> SRAPDQDEIQRLPGLAKQPSFRQYSGYLKGSGSKHLHYWFVESQKDPENSPVVLWLNGGPGCSSLDGLLTEHGPFLVQPDGVTLEYNPYSWNLIANVLYLESPAGVGFSYSDDKFYATNDTEVAQSNFEALQDFFRLFPEYKNNKLFLTGESYAGIYIPTLAVLVMQDPSMNLQGLAVGNGLSSYEQNDNSLVYFAYYHGLLGNRLWSSLQTHCCSQNKCNFYDNKDLECVTNLQEVARIVGNSGLNIYNLYAPCAGGVPSHFRYEKDTVVVQDLGNIFTRLPLKRMWHQALLRSGD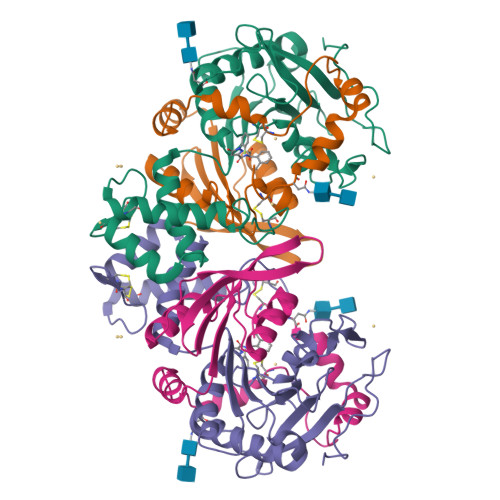KVR;> MDPPCTNTTAASTYLNNPYVRKALNIPEQLPQWDMCNFLVNLQYRRLYRSMNSQYLKLLSSQKYQILLYNGDVDMACNFMGDEWFVDSLNQKMEVQRRPWLVKYGDSGEQIAGFVKEFSHIAFLTIKGAGHMVPTDKPLAAFTMFSRFLNKQPYE>MFENITAAPADPILGLADLFRADERPGKINLGIGVYKDETGKTPVLTSVKKAEQYLLENETTKNYLGIDGIPEFGRCTQELLFGKGSALINDKRARTAQTPGGTGALRVAADFLAKNTSVKRVWVSNPSWPNHKSVFNSAGLEVREYAYYDAENHTLDFDALINSLNEAQAGDVVLFHGCCHNPTGIDPTLEQWQTLAQLSVEKGWLPLFDFARQGFARGLEEDAEGLRAFAAMHKELIVASSYSKNFGLYNERVGACTLVAADSETVDR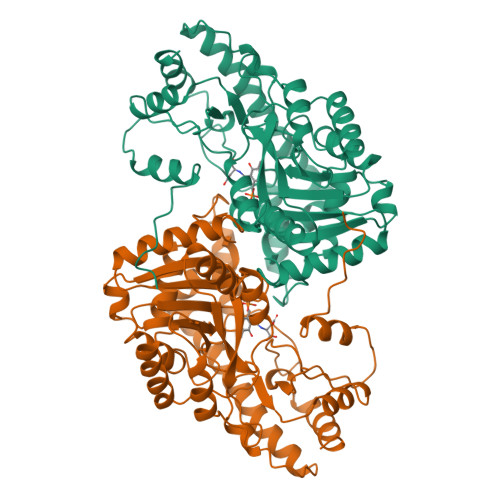AFSQMKAAIRANYSNPPAHGASVVATILSNDALRAIWEQELTDMRQRIQRMRQLFVNTLQEKGANRDFSFIIKQNGMFSFSGLTKEQVLRLREEFGVYAVASGAVNVAGMTPDNMAPLCEAIVAVL[2x]>GRKKIQISRILDQRNRQVTFTKRKFGLMKKAYELSVLCDCEIALIIFNSANRLFQYASTDMDRVLLKYTEYSEPHESRTNTDILETLKRR[4x];>KPRVLFSQAQVYELERRFKQQRYLSAPERDQLASVLKLTSTQVKI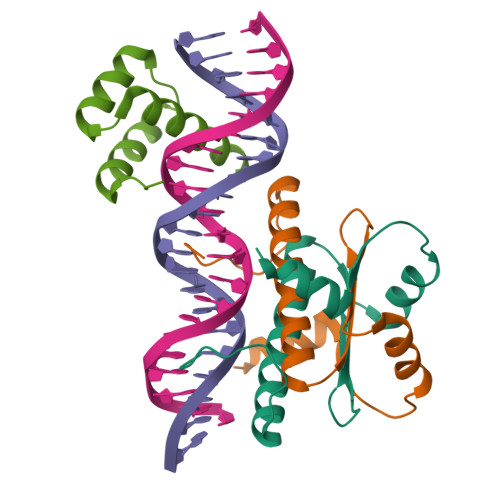WFQNRRYKSKRQ[2x]> MKTQVAIIGAGPSGLLLGQLLHKAGIDNVILERQTPD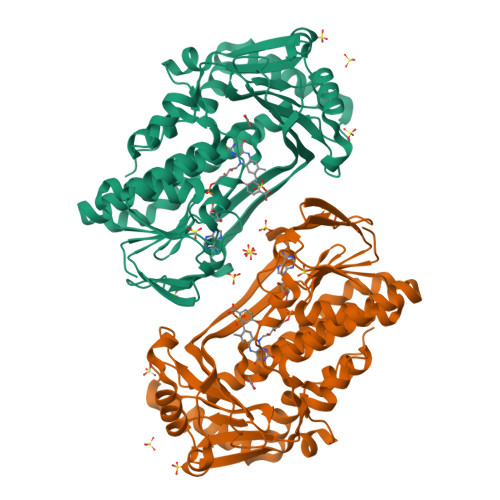YVLGRIRAGVLEQGMVDLLREAGVDRRMARDGLVHEGVEIAFAGQRRRIDLKRLSGGKTVTVYGQTEVTRDLMEAREACGATTVYQAAEVRLHDLQGERPYVTFERDGERLRLDCDYIAGCDGFHGISRQSIPAERLKVFERVYPFGWLGLLADTPPVSHELIYANHPRGFALCSQRSATRSQYYVQVPLSEKVEDWSDERFWTELKARLPSEVAEKLVTGPSLEKSIAPLRSFVVEPMQHGRLFLAGDAAHIVPPTGAKGLNLAASDVSTLYRLLLKAYREGRGELLERYSAICLRRIWKAERFSWWMTSVLHRFPDTDAFSQRIQQTELEYYLGSEAGLATIAENYVGLPYEEIE>[2x]MLLNALASLGHKGIKTLRTFGRAGLMLFNALVGKPEFRKHAPLLVRQLYNVGVLSMLIIVVSGVFIGMVLGLQGYLVLTTYSAETSLGMLVALSLLRELGPVVAALLFAGRAGSALTAEIGLMRATEQLSSMEMMAVDPLRRVISPRFWAGVISLPLLTVIFVAVGIWGGSLVGVSWKGIDSGFFWSAMQNAVDWRMDLVNCLIKSVVFAITVTWISLFNGYDAIPTSAGISRATTRTVVHSSLAVLGLDFVLTALMFGN;>MEQSVANLVDMRDVSFTRGNRCIFDNISLTVPRGKITAIMGPSGIGKTTLLRLIGGQIAPDHGEILFDGENIPAMSRSRLYTVRKRMSMLFQSGALFTDMNVFDNVAYPLREHTQLPAPLLHSTVMMKLEAVGLRGAAKLMPSELSGGMARRAALARAIALEPDLIMFDQPFVGQDPITMGVLVKLISELNSALGVTCVVVSHDVPEVLSIADHAWILADKKIVAHGSAQALQANPDPRVRQFLDGIADGPVPFRYPAGDYHADLLPGS[2x];>MSESLSWMQTGDTLALSGELDQDVLLPLWEMREEAVKGITCIDLSRVSRVDTGGLALLLHLIDLAKKQGNNVTLQGVNDKVYTLAKLYNLPADVLPR[2x];>[6x]MQTKKNEIWVGIFLLAALLAALFVCLKAANVTSIRTEPTYTLYATFDNIGGLKARSPVSIGGVVVGRVADITLDPKTYLPRVTLEIEQRYNHIPDTSSLSIRTSGLLGEQYLALNVGFEDPELGTAILKDGDTIQDTKSAMVLEDLIGQFLYGSKGDDNKNSGDAPAAAPGNNETTEPVGTTK

The IM MlaFEDB complex functions as an ABC transporter to translocate phospholipids between the IM and periplasm. This complex is composed of four components, namely the NBD protein MlaF, the TMD protein MlaE, the phospholipid-binding protein MlaD, and the auxiliary protein MlaB. MlaFEDB is assembled in a stoichiometry of 2:2:6:2 (MlaF:MlaE:MlaD:MlaB). MlaD forms a hexameric disc-shaped ring on top of MlaE, with a central pore lined by hydrophobic residues and has been shown to contain phospholipids.

For cryo-EM studies, the purified MlaFEDB complex with the E170Q mutation (MlaFEQEDB) was incubated with 2 mM ATP-Mg2+ prior to the preparation of cryo-EM specimen. Image processing generated cryo-EM maps of the MlaFEQEDB complex in different conformations (EQtall and EQclose) at resolutions of 4.3 and 3.7 Å, respectively. EQclose structure demonstrates tight closure of ATP-binding sites with the Walker A and signature motifs in close proximity, with a clear ATP-like density in between, which is consistent with an ATP-bound conformation. The structure of EQclose showed tight dimerization of the two MlaF subunits, caused by the trapping of ATP-Mg2+ at the ATP-binding sites. The dimerization of the MlaF engages the CHs between TM2 and TM3 of MlaE, which induces the rearrangement of all TMs. The two TMDs move toward each other. TM1, TM2 and TM5 bend clockwise, when viewed from the front side, to collapse the central phospholipid-binding cavity, and accordingly no bound phospholipids were observed in the collapsed central cavity. The TMD conformational change further induce the movement of MlaD. The MlaD hexametric ring twisted and shifted around 30° as aligned to the nucleotide-free structure. EQclose structure elucidates that the ATP binding-coupled conformational change further collapses the central phospholipid-binding cavity and squeezes out the bound phospholipids.> MESNQEVANPEHYIKHPLQNRWALWFFKNDKSKTWQANLRLISKFDTVEDFWALYNHIQLSSNLMPGCDYSLFKDGIEPMWEDAANARGGRWLITLNKQQRRSDLDRF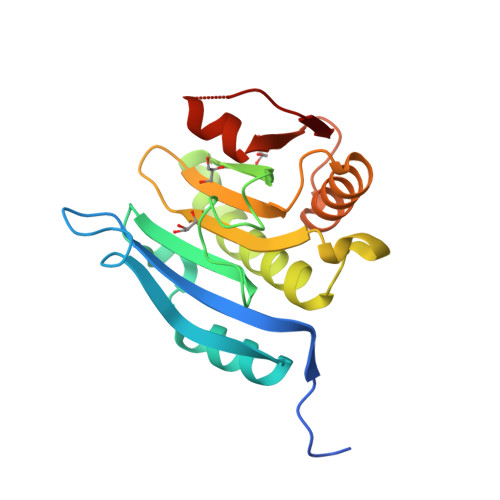WLETLLCLIGESFDDYSDDVCGAVVNVRAKGDKIAIWTTECENREAVTHIGRVYKERLGLPPKIVIGYQSHADTATKSGSTTKNRFVV Another type of cavity, the W191G mutant of Cytochrome c Peroxidase (CcP) is dominated by ion-pair interactions with Asp235. We turned to a mutant of the CcP W191G cavity where the substitution Pro190→Gly has been made and residues Gly192 and Ala193 have been deleted (P190G/W191G/Δ192-3). These residues do not themselves directly interact with ligands but form a capping loop that seals off the original W191G cavity; their deletion opens this cavity to solvent. The closed (W191G) and opened Gateless (P190G/W191G/Δ192-3) cavities in Cytochrome c Peroxidase conserve most features that dominate ligand recognition – the opening of the cavity only deletes residues that are distal to the recognition features of the site, and the crucial cation-recognizing Asp235 is conserved in both (Asp233 in Gateless).

In the docking pose, the ligand contacted Gly178 and Met228 via the benzimidazole nitrogens. In the crystal structure, 22 rotated away from Met228 to interact with Leu177 and Gly178 via one benzimidazole nitrogen and the methylamine tail. The second benzimidazole nitrogen hydrogen-bonded with two ordered waters; these water molecules were not modeled in the docking. Compound 22 interacts with two ordered waters that were not modeled in the docking and the ligand is rotated as compared to the dock pose. Third, structures where we observed a substantial discrepancy between the predicted and experimental ligand poses saw the intervention of new ordered water molecules that we had not anticipated in the docking model. Part of the effects of opening the cavity to bulk solvent appears to be qualitatively captured by a continuum-based electrostatic model in docking, though the role of ordered waters is not, and their effects can be considerable.

> LVHVASVEKGRSYEDFQKVYNAIALKLREDDEYDNYIGYGPVLVRLAWHISGTWDKHDNTGGSYGGTYRFKKEFNDPSNAGLQNGFKFLEPIHKEFPWISSGDLFSLGGVTAVQEMQGPKIPWRCGRVDTPEDTTPDNGRLPDADKDAGYVRTFFQRLNMNDREVVALMGAHALGKTHLKNSGYEGGGANNVFTNEFYLNLLNEDWKLEKNDANNEQWDSKSGYMMLPTDYSLIQDPKYLSIVKEYANDQDKFFKDFSKAFEKLLENGITFPKDAPSPFIFKTLEEQGL(1R,3S,5E,7S,11R,13E,15E,17E,19E,21R,23S,24R,25S)-11,24-dimethyl-1,3,7,21,25-pentakis(oxidanyl)-10,27-dioxabicyclo[21.3.1]heptacosa-5,13,15,17,19-pentaen-9-one 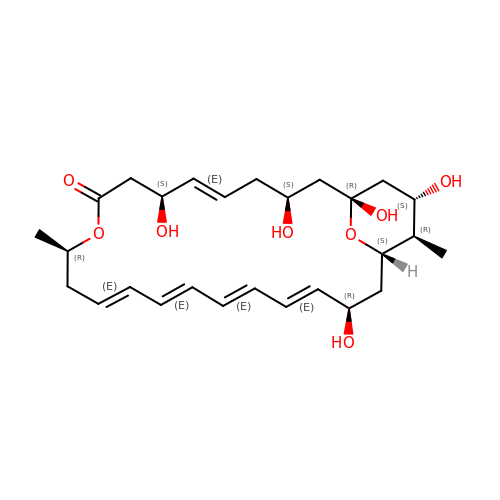| C27 H40 O8 | HPNUEFYWFLZIDL-RYQDMBGZSA-N> MVSATYSVVYETGKKLNSGFDNWGWDSKMSFKDNSLVLTADPDEYGAISLKNLNSNYYGKGGCIYLQVKTETEGLVKVQGVRGYDETEAFNVGSF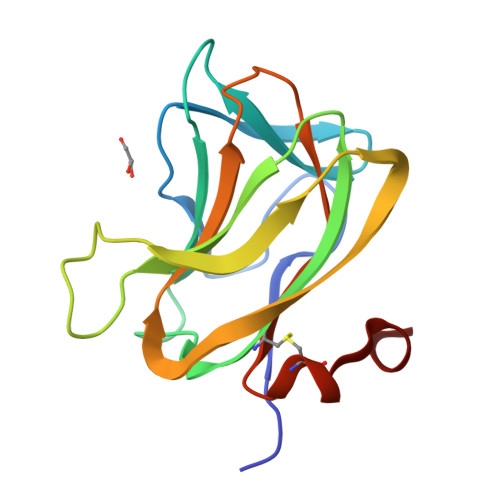RSSSDFTEYKFEVDDEYQFDRIIVQDGPASNIPIYMRYIIYSTGSCDDHILEHHHHHH>MAKDIEISASESKFILEALRQNYRLDGRSFDQFRDVEITFGKEFGDVSVKMGNTKVHCRISCQIAQPYEDRPFEGLFVISTEISPMAGSQFENGNITGEDEVLCSRIIEKSVRRSGALDVEGLCIVAGSKCWAVRADVHFLDCDGGFIDASCIAVMAGLMHFKKPDITVHGEQIIVHPVNEREPVPLGILHIPICVTFSFFNPQDTEENIKGETNSEISIIDATLKEELLRDGVLTVTLNKNREVVQVSKAGGLPMDALTLMKCCHEAYSIIEKITDQILQLLKEDSEKRNKYAAMLTSENAREI[4x];>[4x]GPHMSRLEIYSPEGLRLDGRRWNELRRFESSINTHPHAADGSSYMEQGNNKIITLVKGPKEPRLKSQMDTSKALLNVSVNITKFSKFERSKSSHKNERRVLEIQTSLVRMFEKNVMLNIYPRTVIDIEIHVLEQDGGIMGSLINGITLALIDAGISMFDYISGISVGLYDTTPLLDTNSLEENAMSTVTLGVVGKSEKLSLLLVEDKIPLDRLENVLAIGIAGAHRVRDLMDEELRKHAQKRVSNASAR;>[4x]MAESTTLETIEIHPITFPPEVLARISPELSLQRHLSLGIRPCLRKYEEFRDVAIENNTLSRYADAGNIDTKNNILGSNVLKSGKTIVITSITGGIIEETSAAIKDLDDFGEEELFEVTKEEDIIANYASVYPVVEVERGRVGACTDEEMTISQKLHDSILHSRILPKKALKVKAGVRSANEDGTFSVLYPDELEDDTLNETNLKMKRKWSYVLYAKIVVLSRTGPVFDLCWNSLMYALQSVKLPRAFIDERASDLRMTIRTRGRSATIRETYEIICDQTKSVPLMINAKNIAFASNYGIVELDPECQLQNSDNSEEEEVDIDMDKLNTVLIADLDTEAEETSIHSTISILAAPSGNYKQLTLMGGGAKITPEMIKRSLLLSRVRADDLSTRFNI;>[4x]AASMSVQAEIGILDHVDGSSEFVSQDTKVICSVTGPIEPKARQELPTQLALEIIVRPAKGVATTREKVLEDKLRAVLTPLITRHCYPRQLCQITCQILESGEDEAEFSLRELSCCINAAFLALVDAGIALNSMCASIPIAIIKDTSDIIVDPTAEQLKISLSVHTLALEFVNGGKVVKNVLLLDSNGDFNEDQLFSLLELGEQKCQELVTNIRRIIQDNISPRLVV;>[4x]GPHMSLSVAEKSYLYDSLASTPSIRPDGRLPHQFRPIEIFTDFLPSSNGSSRIIASDGSECIVSIKSKVVDHHVENELLQVDVDIAGQRDDALVVETITSLLNKVLKSGSGVDSSKLQLTKKYSFKIFVDVLVISSHSHPISLISFAIYSALNSTYLPKLISAFDDLEVEELPTFHDYDMVKLDINPPLVFILAVVGNNMLLDPAANESEVANNGLIISWSNGKITSPIRSVALNDSNVKSFKPHLLKQGLAMVEKYAPDVVRSLENL;>MNVQDRRRLLGPAAAKPMAFSNTTTHVPEKKSTDLTPKGNESEQELSLHTGFIENCNGSALVEARSLGHQTSLITAVYGPRSIRGSFTSQGTISIQLKNGLLEKYNTNELKEVSSFLMGIFNSVVNLSRYPKSGIDIFVYLTYDKDLTNNPQDDDSQSKMTSSQISSLIPHCITSITLALADAGIELVDMAGAGEANGTVVSFIKNGEEIVGFWKDDGDDEDLLECLDRCKEQYNRYRDLMISCLMNQET[4x];>[4x]GPDSMSTFIFPGDSFPVDPTTPVKLGPGIYCDPNTQEIRPVNTGVLHVSAKGKSGVQTAYIDYSSKRYIPSVNDFVIGVIIGTFSDSYKVSLQNFSSSVSLSYMAFPNASKKNRPTLQVGDLVYARVCTAEKELEAEIECFDSTTGRDAGFGILEDGMIIDVNLNFARQLLFNNDFPLLKVLAAHTKFEVAIGLNGKIWVKCEELSNTLACYRTIMECCQKNDTAAFKDIAKRQFKEILTVKEE;>TGGRSMSDSQIVTPGELVTDDPIWMRGHGTYFLDNMTYSSVAGTVSRVNRLLSVIPLKGRYAPETGDHVVGRIAEVGNKRWKVDIGGKQHAVLMLGSVNLPGGILRRKSESDELQMRSFLKEGDLLNAEVQSLFQDGSASLHTRSLKYGKLRNGMFCQVPSSLIVRAKNHTHNLPGNITVVLGVNGYIWLRKTSQMDLARDTPSANNSSSIKSTGPTGAVSLNPSITRLEEESSWQIYSDENDPSISNNIRQAICRYANV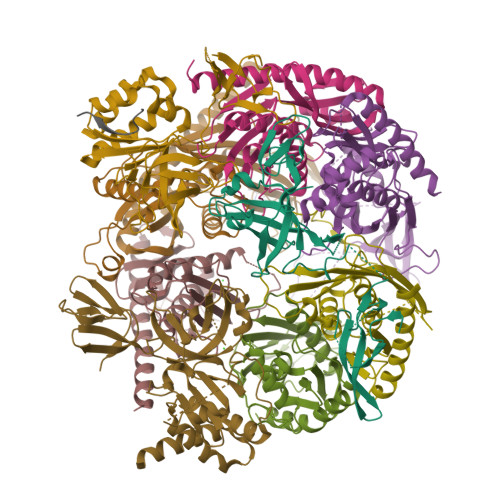IKALAFCEIGITQQRIVSAYEASMVYSNVGELIEKNVMESIGSDILTAEKMRGNGN[4x];>GPHMACNFQFPEIAYPGKLICPQYGTENKDGEDIIFNYVPGPGTKLIQYEHNGRTLEAITATLVGTVRCEEEKKTDQEEEREGTDQSTEEEKSVDASPNDVTRRTVKNILVSVLPGTEKGRKTNKYANNDFANNLPKEGDIVLTRVTRLSLQRANVEILAVEDKPSPIDSGIGSNGSGIVAAGGGSGAATFSVSQASSDLGETFRGIIRSQDVRSTDRDRVKVIECFKPGDIVRAQVLSLGDGTNYYLTTARNDLGVVFARAANGAGGLMYATDWQMMTSPVTGATEKRKCAKPF[4x];>GPDSMSANNGVTGKLSSRVMNMKFMKFGKTDDEESSNSNTPSNINSDVEPIEQKGKLFGLDDSAWDLNSYKDDLKKISGKEKKKVKRVVYKKRPNLIISNVGYSELRKPEGVISGRKTFGDNSDDSGSRKRKFDEGEQNEDEKRDAKDKEFTGSQDDGEDEYDLDKLFKDSIKKKKTNHNGKNKNRNSKK[4x]>GSHMASPNGQTKPLPALKLALEYIVPAMNKHGICVVDDFLGKETGQQIGDEVRALHDTGKFTDGQLVSQKSDSSKDIRGDKITWIEGKEPGCETIG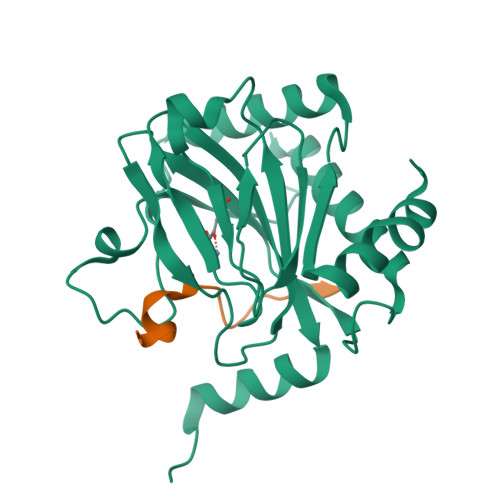LLMSSMDDLIRHCNGKLGSYKINGRTKAMVACYPGNGTGYVRHVDNPNGDGRCVTCIYYLNKDWDAKVSGGILRIFPEGKAQFADIEPKFDRLLFFWSDRRNPHEVQPAYATRYAITVWYFDADERAAAKVKYLTGEKGVRVELNKPSDSVGKDVF[2x];>[2x]DLDLEMLAPYIPMDDDFQL> GPMTTTERPDLAWLDEVTMTQLERNPYEVYERLRAEAPLAFVPVLGSYVASTAEVCREVATSPDFEAVITPAGGRTFGHPAIIGVNGDIHADLRSMVEPALQPAEVDRWIDDLVRPIARRYLERFENDGHAELVAQYCEPVSVRSLGDLLGLQEVDSDKLREWFAKLNRSATNAAVDENGEFANPEGFAEGDQAKAEIRAVVDPLIDKWIEHPDDSAISHWLHDGMPPGQTRDREYIYPTIYVYLLGAMQEPGHGMASTLVGLFSRPEQLEEVVDDPTLIPRAIAEGLRWTSPIWSASARISTKPVTIAGVDLPAGTPVMLSYGSANHDTGKYEAPSQYDLHRPPLPHLAFGAGNHACAGIYFANHVMRIALEELFEAIPNLERDTREGVEFWGWGFRGPTSLHVT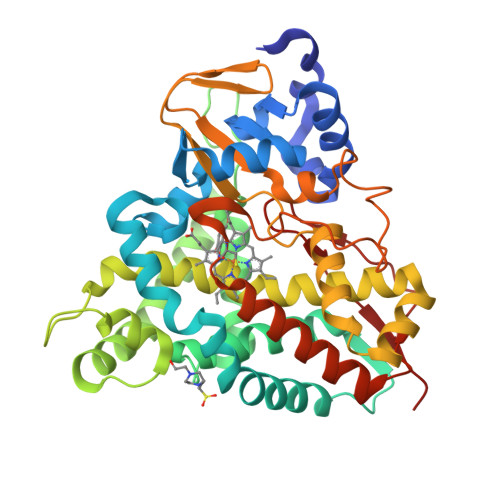WEV>[4x]MDNQKGRISIALLPFLAHGHISPFFELAKQLAKRNCNVFLCSTPINLSSIKDKDSSASIKLVELHLPSSPDLPPHYHTTNGLPSHLMLPLRNAFETAGPTFSEILKTLNPDLLIYDFNPSWAPEIASSHNIPAVYFLTTAAASSSIGLHAFKNPGEKYPFPDFYDNSNIIPEPPSADNMKLLHDFIACFERSCDIILIKSFRELEGKYIDLLSTLSDKTLVPVGPLVQDPMGHNEDPKTEQIINWLDKRAESTVVFVCFGSEYFLSNEELEEVAIGLEISTVNFIWAVRLIEGEKKGILPEGFVQRVGDRGLVVEGWAPQARILGHSSTGGFVSHCGWSSIAESMKFGVPVIAMARHLDQPLNGKLAAEVGVGMEVVRDENGKYKREGIAEVIRKVVVEKSGEVIRRKARELSEKMKEKGEQEIDRAVEELVQICKKKKDEQENLYFQGHHHHHH

Pq3‐O‐UGT2, an important UDP‐dependent glycosyltransferase (UGT), catalyzes the production of Ginsenoside Rg3 and Rd by extending the glycan chain of Ginsenoside Rh2 and F2, respectively, with higher selectivity for F2. Pq3‐O‐UGT2 catalyzes glucose transfer from UDP‐Glucose (UDP‐Glc) to the C2‐OH of the C3‐glucose of Ginsenoside Rh2 and F2, respectively. In this study, we elucidated the crystal structures of both apo Pq3‐O‐UGT2 and its complexes with Ginsenoside Rh2 and F2, revealing the acceptor recognition mechanisms of Pq3‐O‐UGT2. The NTD contains a seven‐stranded parallel β‐sheet sandwiched by seven helices, while the CTD comprises a 6‐stranded parallel β‐sheet flanked by 6 helices.

To elucidate the underlying molecular mechanisms, we solved crystal structures of apo Pq3‐O‐UGT2 and its complex with Rh2 at resolutions of 2.9 and 3.5 Å, respectively. The apo structure adopted a P1 space group with four molecules in the asymmetric unit, while the Pq3‐O‐UGT2‐Rh2 complex exhibited a P212121 space group with two molecules in the asymmetric unit. PISA analysis indicated the absence of higher‐order assemblies in solution, consistent with the monomeric state observed via gel filtration. The C‐terminal helix (Cα7) extends from the CTD to the NTD, stabilizing the two‐lobe structure of Pq3‐O‐UGT2. Alignment of the AlphaFold2 predicted Pq3‐O‐UGT2 structure with each of the four molecules in the asymmetric unit suggests that the absence of density in Nβ3‐Nα3, Nα5‐Nα6, and Cβ2‐Cα3 is likely due to spatial conflict during crystal packing, while the missing density of the intermediate loop may result from flexibility. Comparison of the apo and complex structures reveals significant conformational changes in the NTD.>[2x]RSHHHHHHGDAAQKTDTSHHDQDHPTFNKITPNLAEFAFSLYRQLAHQSNSTNIFFSPVSIATAFAMLSLGTKADTHDEILE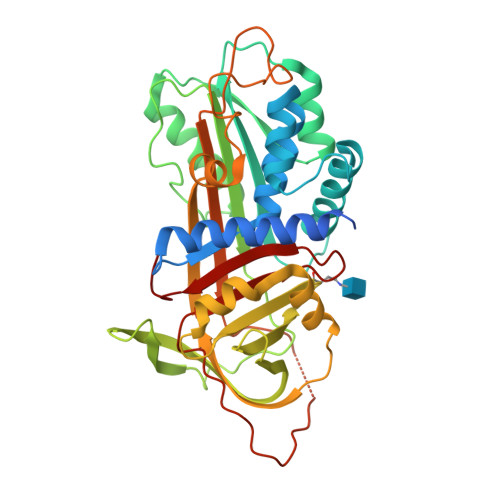GLNFNLTEIPEAQIHEGFQELLRTLNQPDSQLQLTTGNGLFLSEGLKLVDKFLEDVKKLYHSEAFTVNFGDTEEAKKQINDYVEKGTQGKIVDLVKELDRDTVFALVNYIFFKGKWERPFEVKDTEEEDFHVDQVTTVKVPMMKRLGMFNIQHCKKLSSWVLLMKYLGNATAIFFLPDEGKLQHLENELTHDIITKFLENEDRRSASLHLPKLSITGTYDLKSVLGQLGITKVFSNGADLSGVTEEAPLKLSKAVHKAVLTIDKKGCEAAGAMFLEAIPRSIPPEVKFNKPFVFLMIEQNTKSPLFMGKVVNPTQK>[5x]GDRVADVIESSIGDSVSRALTHALPAPTGQNTQVSSHRLDTGKVPALQAAEIGASSNASDESMIETRCVLNSHSTAETTLDSFFSRAGLVGEIDLPLEGTTNPNGYANWDIDITGYAQMRRKVELFTYMRFDAEFTFVACTPTGEVVPQLLQYMFVPPGAPKPDSRESLAWQTATNPSVFVKLSDPPAQVSVPFMSPASAYQWFYDGYPTFGEHKQEKDLEYGACPNNMMGTFSVRTVGTSKSKYPLVVRIYMRMKHVRAWIPRPMRNQNYLFKANPNYAGNSIKPTGASRTAITTL;>GFPTELKPGTNQFLTTDDGVSAPILPNFHPTPCIHIPGEVRNLLELCQVETILEVNNVPTNATSLMERLRFPVSAQAGKGEL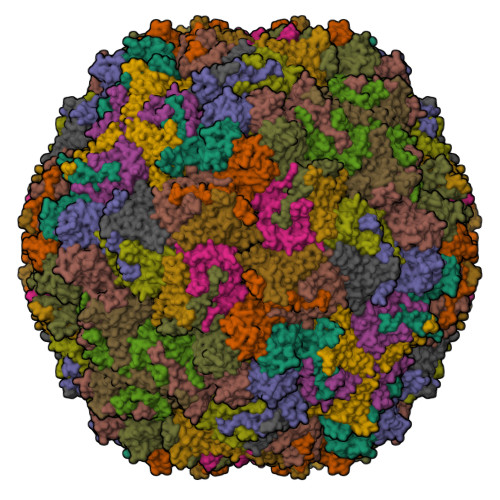CAVFRADPGRSGPWQSTLLGQLCGYYTQWSGSLEVTFMFTGSFMATGKMLIAYTPPGGPLPKDRATAMLGTHVIWDFGLQSSVTLVIPWISNTHYRAHARDGVFDYYTTGLVSIWYQTNYVVPIGAPNTAYIIALAAAQKNFTMQLCKDASDILQTGTIQ[5x];>[5x]MGSQVSTQRSGSHENSNSATEGSTINYTTINYYKDSYAATAGKQSLKQDPDKFANPVKDIFTEMAAPLKSPSAEACGYSDRVAQLTIGNSTITTQEAANIIVGYGEWPSYCSDSDATAVDKPTRPDVSVNRFYTLDTKLWEKSSKGWYWKFPDVLTETGVFGQNAQFHYLYRSGFCIHVQCNASKFHQGALLVAVLPEYVIGTVAGGTGTEDSHPPYKQTQPGADGFELQHPYVLDAGIPISQLTVCPHQWINLRTNNCATIIVPYINALPFDSALNHCNFGLLVVPISPLDYDQGATPVIPITITLAPMCSEFAGLRQAVTQ> GHMSGGGEQADILPANYVVKDRWKVLKKIGGGGFGEIYEAMDLLTRENVALKVESAQQPKQVLKMEVAVLKKLQGKDHVCRFIGCGRNEKFNYVVMQLQGRNLADLRRSQPRGTFTLSTTLRLGKQILESIEAIHSVGFLHRDIKPSNFAMGRLPSTYRKCYMLDFGLARQYTNTTGDVRPPRNVAGFRGTVRYASVNAHKNREMGRHDDLWSLFYMLVEFAVGQLPWRKIKD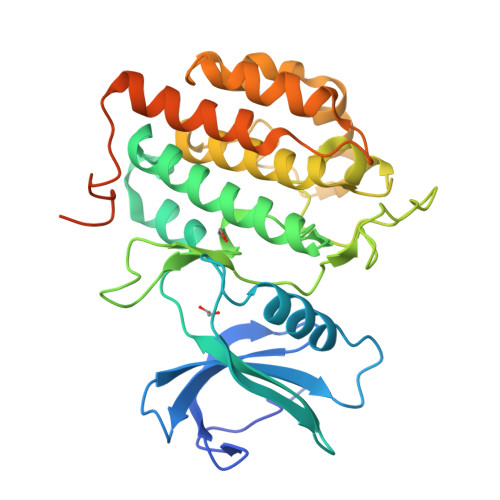KEQVGMIKEKYEHRMLLKHMPSEFHLFLDHIASLDYFTKPDYQLIMSVFENSMKERGIAENEAFDWEKAGTDALLSTSTSTPPQQNTRQTAAMFGVVNV> MQRASRLKRELHMLATEPPPGITCWQDKDQMDDLRAQILGGANTPYEKGVFKLEVIIPERYPFEPPQIRFLTPIYHPNIDSAGRICLDVLKLPPKGAWRPSLNIATVLTSIQLLMSEPNPDDPLMADISSEFKYNKPAFLKNARQWTEKHARQKQKADEEEM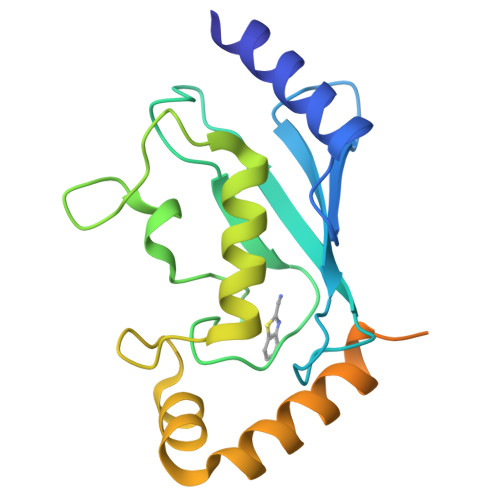LDNLPEAGDSRVHNSTQKRKASQLVGIEKKFHPDV> AANDNNVEWNGLFHDQGPLFDNAPEPTSTQSVTLKLRTFKGDITSANIKYWDTADNAFHWVPMVWDSNDPTGTFDYWKGTIPASPSIKYYRFQINDGTSTAWYNGNGPSSTEPNADDFYIIPNFKTPDWLKNGVMYQIFPDRFYNGDSSNDVQTGSYTYNGTPTEKKAWGSSVYADPGYDNSLVFFGGDLAGIDQKLGYIKKTLGANILYLNPIFKAP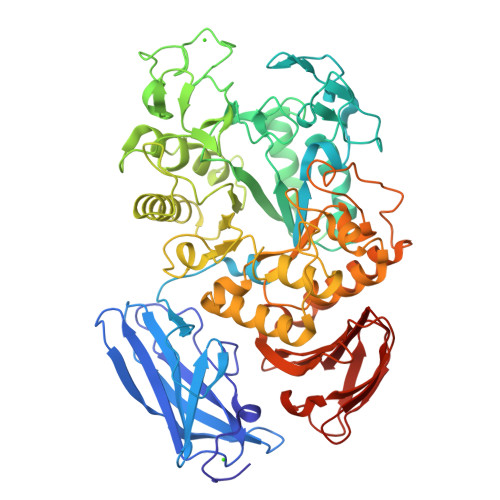TNHKYDTQDYMAVDPAFGDNSTLQTLINDIHSTANGPKGYLILDGVFNHTGDSHPWFDKYNNFSSQGAYESQSSPWYNYYTFYTWPDSYASFLGANSLPKLNYGNSGSAVRGVIYNNSNSVAKTYLNPPYSVDGWRLDAAQYVDANGNNGSDVTNHQIWSEFRNAVKGVNSNAAIIGEYWGNANPWTAQGNQWDAATNFDGFTQPVSEWITGKDYQNNSASISTTQFDSWLRGTRANYPTNVQQSMMNFLSNHDITRFATRSGGDLWKTYLALIFQMTYVGTPTIYYGDEYGMQGGADPDNRRSFDWSQATPSNSAVALTQKLITIRNQYPALRTGSFMTLITDDTNKIYSYGRFDNVNRIAVVLNNDSVSHTVNVPVWQLSMPNGSTVTDKITGHSYTVQNGMVTVAVDGHYGAVLAQ> GSGAPPTIQQPSMSSAVALLGQDVDFTCIVNDLGSHMVAFVKADSPPRLLSFDEKVFRRRNKYELKPRIGDLHNEWVLTIKNVQESDRGNYSCQINTEPITLSTGELDVK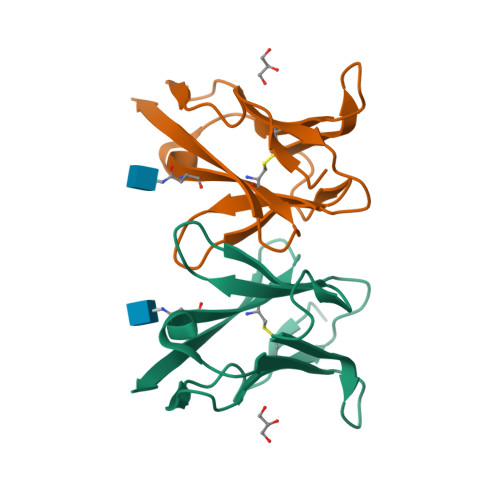VPHHHHHH> MKLVGSYTSPFVRKL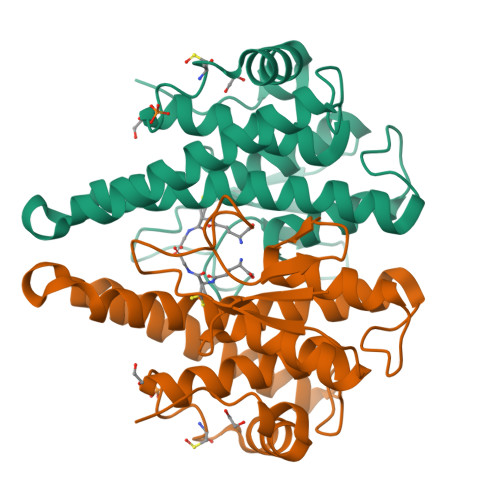SILLLEKGITFEFINELPYNADNGVAQFNPLGKVPVLVTEEGECWFDSPIIAEYIELMNVAPAMLPRDPLESLRVRKIEALADGIMDAGLVSVREQARPAAQQSEDELLRQREKINRSLDVLEGYLVDGTLKTDTVNLATIAIACAVGYLNFRRVAPGWCVDRPHLVKLVENLFSRESFARTEPPKA>[2x]MDVQLPYNVKIEAFEGPLDLLLHLINRYEIDIYDIPVAQITEQYMAYIHAMQELELDIASEYLVMAATL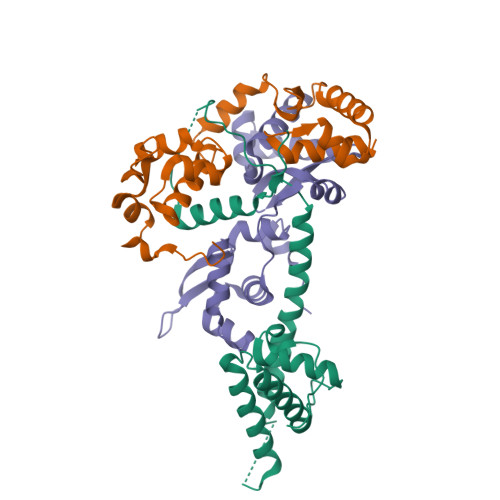LAIKSKMLLPPSNEEAVDGDIEWGDDGDPREELTQRLLEYKKFKEAARELKRREEERALLFTKPPSDLSAYADEKKAAPLDVNVYDMLGALSKLLRRKKLQKPMR;>[4x]GSHMGALKPAKAIVEALLFAAGDEGLSLSQIAAVLEVSELEAKAVIEELQQDCRREERGIQLVELGGVFLLATKKEHAPYLKKLVEAPGASPLSQAALETLAIIAYRQPITRAEIEEIRGVKSDKPLQTLMARALIKEVGRAEGTGRPILYGTTPEFLDYFGLKTLEELPPLPEWADDGESERE> SMGVNATQINEELYRLLEDTEILNQEITEGLLKGFEVPDAGVAIQLSKRDVVYPARILIIVLSE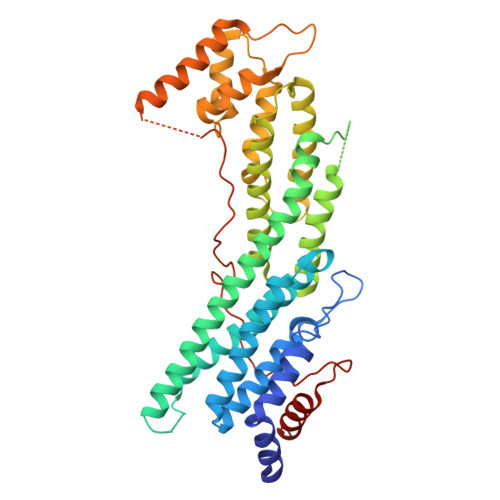MWRFGLTKQSESFLAQVLTTIQKVVTQLKGNDLIPSGVFWLANVRELYSFVVFALNSILTEETFKNGMTDEEYKEYVSLVTELKDDFEALSYNIYNIWLKKLQKQLQKKAINAVVISESLPGFSAGETSGFLNKIFANTEEYTMDDILTFFNSIYWCMKSFHIENEVFHAVVTTLLNYVDAICFNELIMKRNFLSWKRGLQLNYNVTRLEEWCKTHGLTDGTECLQHLIQTAKLLQVRKYTIEDIDILRGICYSLTPAQLQKLISQYQVADYESPIPQEILRYVADIVKKEAALSSSGNDSKGHEHSSSIFITPETGPFTDPFSLIKTRKFDQVEAYIPAWLSLPSTKRIVDLVAQQVVQDGH>TTCCGCCGC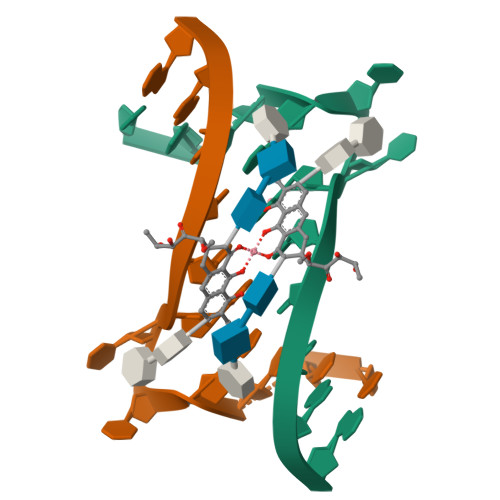CGAA[2x]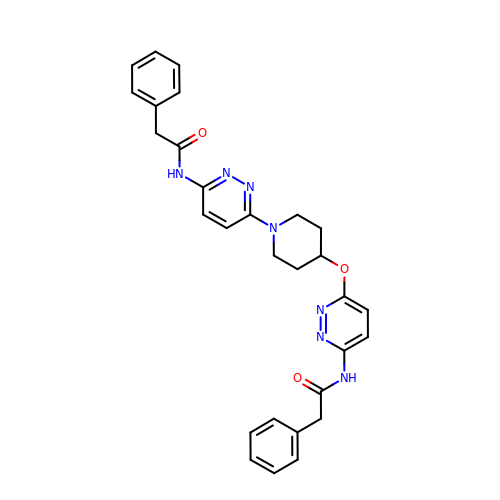2-phenyl-N-{6-[4-({6-[(phenylacetyl)amino]pyridazin-3-yl}oxy)piperidin-1-yl]pyridazin-3-yl}acetamide | C29 H29 N7 O3 | IDGBGPKCEIHLHR-UHFFFAOYSA-N>[2x]IDPFTFEKMVPVSVQQSLAAYNQRKADLVNRSIAQMREATTLANGVLASLNLPAAIEDVSGDTVPQSILTKSRSVIEQGGIQTVDQLIKELPELLQRNREILDESLRLLDEEEATDNDLRAKFKERWQRTPSNELYKPLRAEGTNFRTVLDKAVQADGQVKECYQSHRDTIVLLCKPEPELNAAIPSANPAKTMQGSEVVNVLKSLLSNLDEVKKEREGLENDLKSVN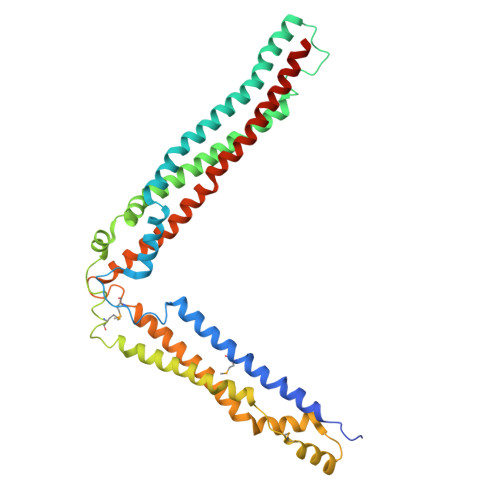FDMTSKFLTALAQDGVINEEALSVTELDRVYGGLTTKVQESLKKQEGLLKNIQVSHQEFSKMKQSNNEANLREEVLKNLATAYDNFVELVANLKEGTKFYNELTEILVRFQNKCSDIVFARKTERRDELLKD> MSDTMVVNGSGGVPAFLFSGSTLSSYRPNFEANSIT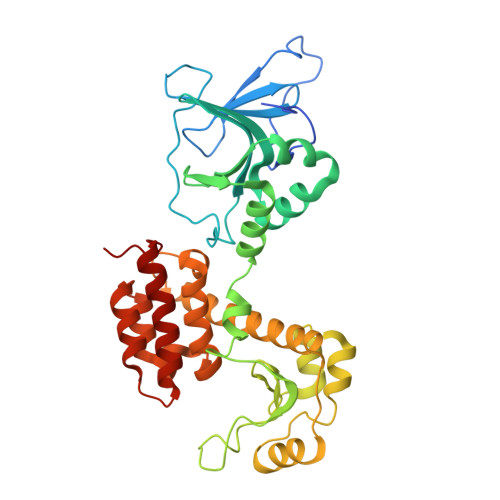IALPHYVDLPGRSNFKLMYIMGFPIDTEMEKDSEYSNKIRQESKISKTEGTVSYEQKITVETGQEKDGVKVYRVMVLEGTIAESIEHLDKKENEDILNNNRNRIVLADNTVINFDNISQLKEFLRRSVNIVDHDIFSSNGFEGFNPTSHFPSNPSSDYFNSTGVAFGSGVDLGQRSKQDLLNDGVPQYIADRLDGYYMLRGKEAYDKVRTAPLTLSDNEAHLLSNIYIDKFSHKIEGLFNDANIGLRFSDLPLRTRTALVSIGYQKGFKLSRTAPTVWNKVIAKDWNGLVNAFNNIVDGMSDRRKREGALVQKDIDSGLLKLH ADENOSINE-5'-[LYSYL-PHOSPHATE] 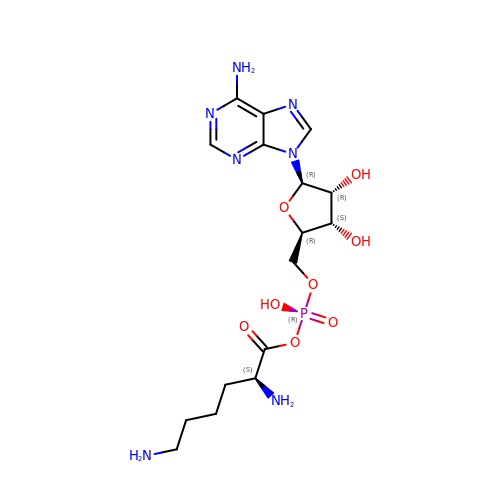| C16 H26 N7 O8 P | RZWIOOBQBMRZTQ-OPYVMVOTSA-N> ADPGTSECSVIGYNAICINRGLHQVPELPAHVNYVDLSLNSIAELNETSFSRLQDLQFLKVEQQTPGLVIRNNTFRGLSSLIILKLDYNQFLQLETGAFNGLANLEVLTLTQCNLDGAVLSGNFFKPLTSLEMLVLRDNNIKKIQPASFFLNMRRFHVLDLTFNKVKSICEEDLLNFQGKHFTLLRLSSITLQDMNEYWLGWEKCGNPFKNTSITTLDLSGNGFKESMAKRFFDAIAGTKIQSLILSNSYN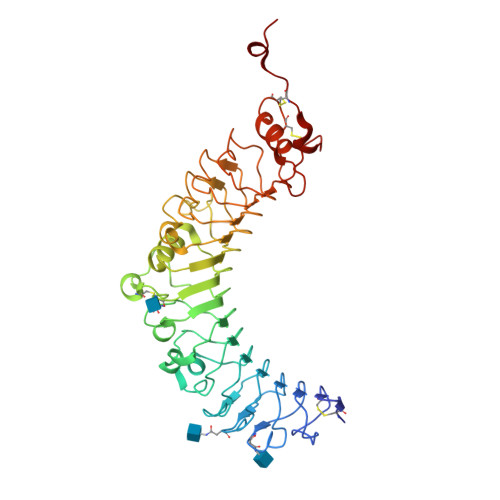MGSSFGHTNFKDPDNFTFKGLEASGVKTCDLSKSKIFALLKSVFSHFTDLEQLTLAQNEINKIDDNAFWGLTHLKELALDTNQLKSVPDGIFDRLTSLQKIWLHTNPWDCSCPRIDYLSRWLNKNSQKEQGSAKCSGSGKPVRSIICPTSASLVPR>[2x]MNSKCHCVILNDGNFIPVLGFGTALPLECPKSKAKELTKIAIDAGFHHFDSASVYNTEDHVGEAIRSKIADGTVRREDIFYTSKVWCTSLHPELVRASLERSLQKLQFDYVDLYLIHYPMALKPGEENFPVDEHGKLIFDRVDLCATWEAMEKCKDAGLTKSIGVSNFNYRQLEMILNKPGLKYKPVCN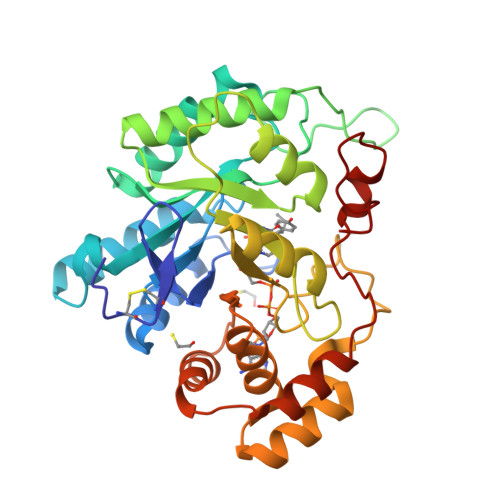QVECHPYLNQMKLLDFCKSKDIVLVAYGVLGTQRYPPWVDQNSPVLLDEPVLGSMAKKYNRTPALIALRYQLQRGIVVLNTSLKEERIKENMQVFEFQLSSEDMKVLDGLNRNMRYIPAAIFKGHPNWPFLDEY>[2x]MSREEVESLIQEVLEVYPEKARKDRNKHLAVNDPAVTQSKKCIISNKKSQPGLMTIRGCAYAGSKGVVWGPIKDMIHISHGPVGCGQYSRAGRRNYYIGTTGVNAFVTMNFTSDFQEKDIVFGGDKKLAKLIDEVETLFPLNKGISVQSECPIGLIGDDIESVSKVKGAELSKTIVPVRCEGFRGVSQSLGHHIANDAVRDWVLGKRDEDTTFASTPYDVAIIGDYNIGGDAWSSRILLEEMGLRCVAQ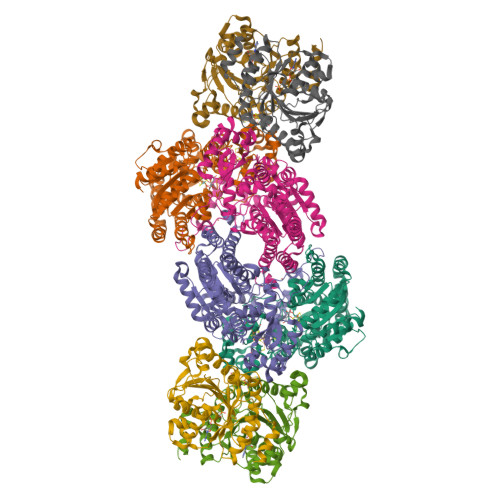WSGDGSISEIELTPKVKLNLVHCYRSMNYISRHMEEKYGIPWMEYNFFGPTKTIESLRAIAAKFDESIQKKCEEVIAKYKPEWEAVVAKYRPRLEGKRVMLYIGGLRPRHVIGAYEDLGMEVVGTGYEFAHNDDYDRTMKEMGDSTLLYDDVTGYEFEEFVKRIKPDLIGSGIKEKFIFQKMGIPFRQMHSWDYSGPYHGFDGFAIFARDMDMTLNNPCWKKLQAPWE;>SQQVDKIKASYPLFLDQDYKDMLAKKRDGFEEKYPQDKIDEVFQWTTTKEYQELNFQREALTVNPAKACQPLGAVLCALGFEKTMPYVHGSQGCVAYFRSYFNRHFREPVSCVSDSMTEDAAVFGGQQNMKDGLQNCKATYKPDMIAVSTTCMAEVIGDDLNAFINNSKKEGFIPDEFPVPFAHTPSFVGSHVTGWDNMFEGIARYFTLKSMDDKVVGSNKKINIVPGFETYLGNFRVIKRMLSEMGVGYSLLSDPEEVLDTPADGQFRMYAGGTTQEEMKDAPNALNTVLLQPWHLEKTKKFVEGTWKHEVPKLNIPMGLDWTDEFLMKVSEISGQPIPASLTKERGRLVDMMTDSHTWLHGKRFALWGDPDFVMGLVKFLLELGCEPVHILCHNGNKRWKKAVDAILAASPYGKNATVYIGKDLWHLRSLVFTDKPDFMIGNSYGKFIQRDTLHKGKEFEVPLIRIGFPIFDRHHLHRSTTLGYEGAMQILTTLVNSILERLDEETRGMQATDYNHDLVR[2x];>AMRQCAIYGKGGIGKSTTTQNLVAALAEMGKKVMIVGCDPKADSTRLILHSKAQNTIMEMAAEAGTVEDLELEDVLKAGYGGVKCVESGGPEPGVGCAGRGVITAINFLEEEGAYEDDLDFVFYDVLGDVVCGGFAMPIRENKAQEIYIVCSGEMMAMYAANNISKGIVKYANSGSVRLGGLICNSRNTDREDELIIALANKLGTQMIHFVPRDNVVQRAEIRRMTVIEYDPKAKQADEYRALARKVVDNKLLVIPNPITMDELEELLMEFGIMEV[4x]> MNLEGL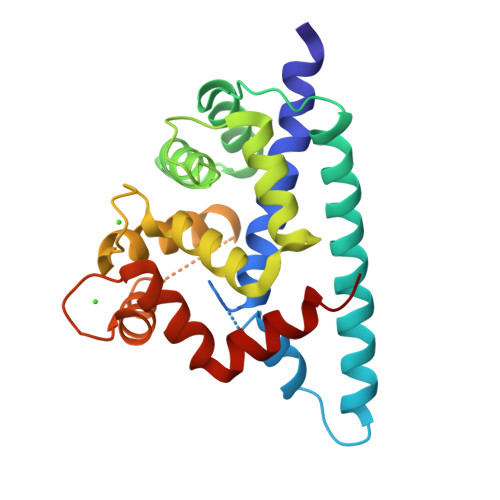EMIAVLIVIVLFVKLLEQFGLIEAGLEDSVEDELEMATVRHRPEALELLEAQSKFTKKELQILYRGFKNECPSGVVNEETFKEIYSQFFPQGDSTTYAHFLFNAFDTDHNGAVSFEDFIKGLSILLRGTVQEKLNWAFNLYDINKDGYITKEEMLDIMKAIYDMMGKCTYPVLKEDAPRQHVETFFQKMDKNKDGVVTIDEFIESCQKDENIMRSMQLFENVI> MAGVKNSIIWFRKGLRLHDNPALLEACKDAKHVYPVFVLDPHFLQQSSYKVSVNRYNFLLESLEDLQRSFQARGSRLLVLRGKPEEVFPRVFREWGVTQLCFEHDTEPYAKVRDA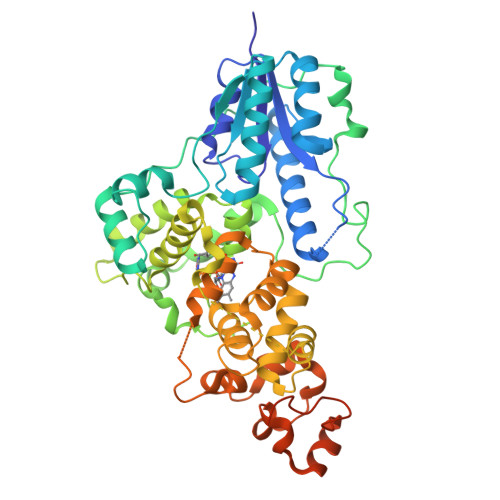AVRRLAAEAGVEVVTPISHTLYDTDMLVARNGGAAPLTMQSFTKLVDRVGDPPAPAPDPPAAMPPPAEDMPSAAPAATGVPTWQEVGFKEPPLTVFKGGETEALARLEAAFQDPKWVAGFQKPDTDPSAWEKPATTVLSPYLKFGCLSARLFHARLLEVYRRHPAHSQPPVSLRGQLLWREFFYTVGSTTPNFHRMAGNPVCKQIDWDDNPEFLAAWREARTGFPWIDAIMTQLVTWGWMHHLARHSVACFLTRGDLYVSWERGMEVFEEHLIDQDHYLNAANWMWLSASAFFSQYFRVYSPVVFGKKYDPEGRFIRKFLPVLKDMPAKYIYEPWTAPLEVQRKAGCVVGRDYPAPIVDHAVASKACIARMAAAYRRSKGEKLAAALEHHHHHH> MDFLRNLFSQTLSLGSQKERLLDELTLEGVARYMQSERCRRVICLVGAGISTSAGIPDFRSPSTGLYDNLEKYHLPYPEAIFEISYFKKHPEPFFALAKELYPGQFKPTICHYFMRLLKDKGLLLRCYTQNIDTLERIAGLEQEDLVEAHGTFYTSHCVSASCRHEYPLSWMKEKIFSEVTPKCEDCQSLVKPDIVFFGESLPARFFSCMQSDFLKVDLLLVMGTSLQVQPFASLISKAPLSTPRL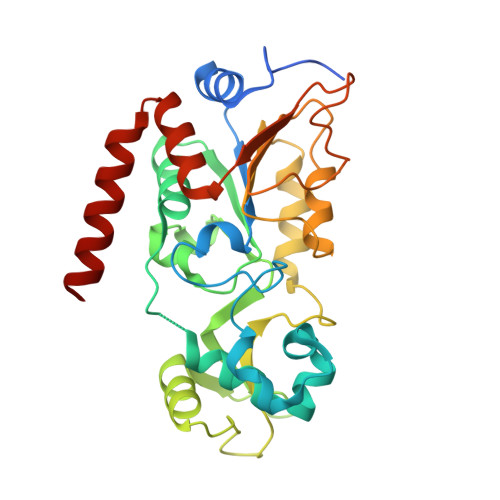LINKEKAGQSDPFLGMIMGLGGGMDFDSKKAYRDVAWLGECDQGCLALAELLGWKKELEDLVRREHASIDAQS> MSRSKRDNNFYSVEIGDSTFTVLKRYQNLKPIGSGAQGIVCAAYDAILERNVAIKKLSRPFQNQTHAKRAYRELVLMKCVNHKNIIGLLNVFTPQKSLEEFQDVYIVMELMDANLCQVIQMELDHERMSYLLYQM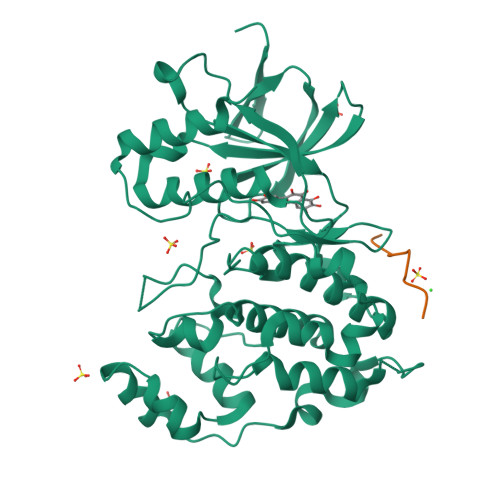LCGIKHLHSAGIIHRDLKPSNIVVKSDCTLKILDFGLARTAGTSFMMTPEVVTRYYRAPEVILGMGYKENVDIWSVGCIMGEMIKGGVLFPGTDHIDQWNKVIEQLGTPCPEFMKKLQPTVRTYVENRPKYAGYSFEKLFPDVLFPADSEHNALKASQARDLLSKMLVIDASKRISVDEALQHPYINVWYDPSEAEAPPPKIPDKQLDEREHTIEEWKELIYKEVMDLPKRPTTLNLFHHHHHH;> RPKRPTTLNLF> SNAMPKERVDVLAYKQGLFETREQAKRGVMAGLVVNVINGERYDKPGEKIDDGTELKLKGEKLRYVSRGGLKLEKALAVFNLSVEDMITIDIGASTGGFTDVMLQNGAKLVYAVDVGTNQLVWKLRQDDRVRSMEQYNFRYAEPVDFTEGLPSFASIDVSFISLNLILPALAKILVDGGQVVALVKPQFEAGREQIGKNGIVRESSIHEKVLET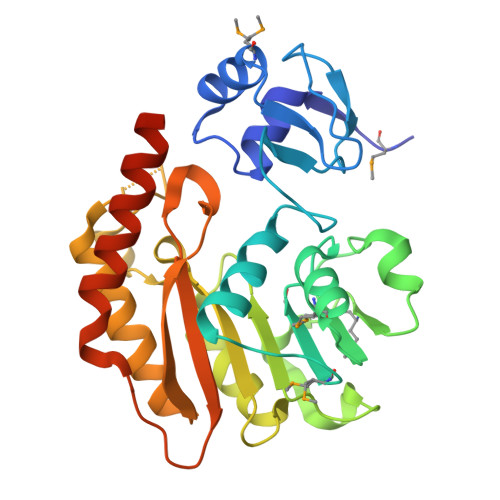VTAFAVDYGFSVKGLDFSPIQGGHGNIEFLAHLEKTDSPQNDVPTSIKEVVAQAHKEFKKNEEERSFGVNPKDCPRK Tyrosinases (TYRs, EC 1.14.18.1 and EC 1.10.3.1) and catechol oxidases (COs, EC 1.10.3.1) are type III copper‐containing metalloenzymes that constitute the class of polyphenol oxidases (PPOs). More specifically, plant PPOs are expressed as pro‐enzymes (55–65 kDa) consisting of an enzymatically active (40–45 kDa) and a C‐terminal domain (15–19 kDa). The C‐terminal domain plays a significant role in the regulation of the enzyme activity inside the cell by shielding the catalytic pocket of the active centre, and in addition it provides an indispensable motif for the accurate folding of the active domain. Herein, we investigated the activation of PPO1 from Malus domestica (MdPPO1) and present a novel activation mode for plant PPOs driven by self‐cleavage, which is independent of external proteases or any other harsh conditions (e.g., SDS).

Therefore, it was suspected that the pro‐enzyme undergoes self‐cleavage, severing the C‐terminal domain from the pro‐enzyme. We recently observed a similar process in apricot PPO, where the enzyme was spontaneously activated upon prolonged storage. The assumed self‐cleavage of MdPPO1 was confirmed by SDS‐PAGE of pro‐enzyme solutions incubated at 4 °C for 20 days, indicating the activation of the pro‐enzyme into its separated active and C‐terminal domains (see the Supporting Information for experimental details). The cleavage site was determined by high‐resolution electrospray ionization mass spectrometry (ESI‐MS), which showed that the protein is not just cleaved at one single peptide bond but rather within a sequence of four contiguous peptide bonds (Ser 366–Ser 367–Ser 368–Lys 369–Val 370). The crystal structure of the Ccleaved‐domain starts at residue Lys 369 and ends at Ser 504, indicating that the C‐terminal domain remains stable upon self‐cleavage. Structural analysis of the separated C‐terminal domains, Ccleaved and Csole, revealed a metal‐binding site. The bound metal was identified as Ca2+ based on the composition of the used expression media and buffers, the interacting amino acids, the binding geometry, and the presence of anomalous signal. This binding site is absent in the C‐terminal domain still attached to the pro‐enzyme. Interestingly, the enzyme retained its latency even after complete cleavage as it did not show any activity on mono‐ or diphenolic substrates. Thus it seems that the C‐terminal domain stays attached to the main domain, presumably because of strong electrostatic interactions between the two domains as indicated by PISA21 analysis (33 hydrogen bonds and 13 salt bridges). It was concluded that the observed cleavage converts the pro‐enzyme into a pre‐active stage that still requires the spatial removal of the C‐terminal domain (e.g., by SDS or high salt concentrations) in order to achieve full enzymatic activity.

> KVVAGTEFPISLGSKISTVVKRPKQKKRSKKAKEDEEEILVIEGIEFDRDVAVKFDVYVNDVDDLPSGPDKTEFAGSFVSVPHSHKHKKKMNTILRLGLTDLLEEIEAEDDDSVVVTLVPKFGAVKIGGIKIEFAS> KLSLQDVAELIRARACQRVVVMVGAGI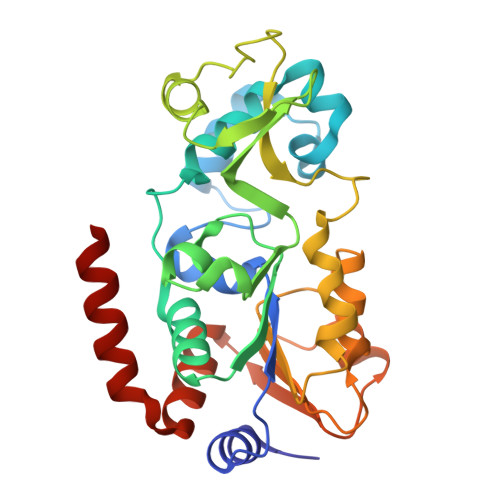STPSGIPDFRSPGSGLYSNLQQYDLPYPEAIFELPFFFHNPKPFFTLAKELYPGNYKPNVTHYFLRLLHDKGLLLRLYTQNIDGLERVSGIPASKLVEAHGTFASATCTVCQRPFPGEDIRADVMADRVPRCPVCTGVVKPDIVFFGEPLPQRFLLHVVDFPMADLLLILGTSLEVEPFASLTEAVRSSVPRLLINRDLVGPLAWHPRSRDVAQLGDVVHGVESLVELLGWTEEMRDLVQRETGKLD>[6x]MKPPSSIQ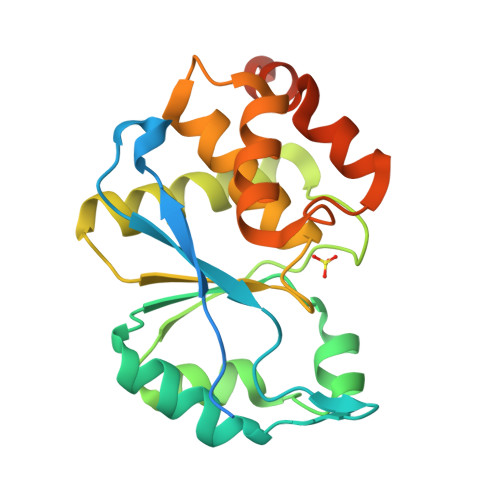TSEFDSSDEEPIEDEQTPIHISWLSLSRVNCSQFLGLCALPGCKFKDVRRNVQKDTEELKSCGIQDIFVFCTRGELSKYRVPNLLDLYQQCGIITHHHPIADGGTPDIASCCEIMEELTTCLKNYRKTLIHSYGGLGRSCLVAACLLLYLSDTISPEQAIDSLRDLRGSGAIQTIKQYNYLHEFRDKLAAHLSSRDSQSRSVSR> PKHLEVYKCTHCGNIVEVLHGGGAELVCCGEPMKHMVEGST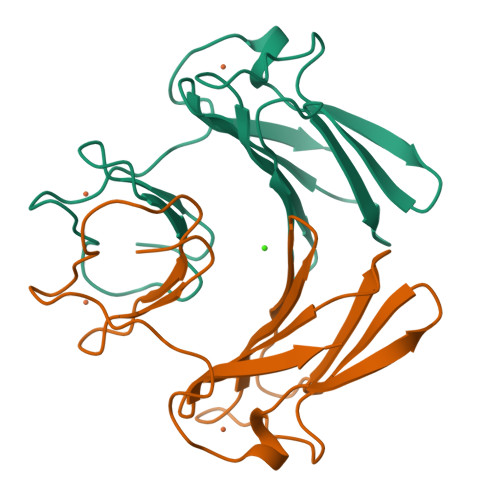DGAMEKHVPVIEKVDGGYLIKVGSVPHPMEEKHWIEWIELLADGRSYTKFLKPGDAPEAFFAIDASKVTAREYCNLHGHWKAEN> GETGQLIKDTIKNTVENTVESTHSISTEATPALQAAETGATSNASDESMIETRNVVNTHGVAETSLEGFYGRAGLVAMFTTEGGIRSWYINFGKYVQLRAKLELLTYARFDVEFTIVAQVVDEQAKVKDFNVDYQVMYVPPGASAPDGQDSFQWQSSCNPSVISNTGLPPARVSVPFMSSANAYSFSYDGYIQFGDTSSSSYGILPIHYLGQLVVRTCEDLDSARLRVRIYAKPKHMRGWIPRSPRMRPYVSRFTGIYTDAPSFCVNRESITTAG;> SAEACGYSDRVAQLTLGNSTITTQEAANIVVAYGRWPSGLRDTDATAVDKPTQPGVSAERFYTLPSVQWTTSFTGHYWKLPDALSDLGLFGQNLQFHYLYRGGWAIHVQCNATKFHQGTLLVVAVPEHKIQAQSNPSFGRTNPGEAGAACQFPFTFEDGTALGNALIYPHQWINLRTNNSATLVLPYVNAIPMDSGIKHNNWTLLVIPIVPLEYAVGATTFVPITVTIAPMCTEYNGLRAAVTQ;> GCPTLYTPGSGQFLTTDDFQTPCMLPKFQPTPVIDIPGEVKNFLEVIQVESLVEINNVSGVEGVARYRIPLNVQDAMDGQIMAVRVDPGADGPMQSTLLGVFTRYYTQWSGSLDFTFMFCGTFMTTGKVIIAYTPPGGDQPGSRQQAMLGTHVVWDFGLQSSITLVVPWISSGHFRGTSLDNTIYKYRYYEAGYITMWYQTNMVVPPNFPTEASILMFVAAQPNFSLRILKDRPDITQVASLQ;> MGAQLSKNTAGSHTTGTYATGGSSIHYTNINYYENAASNSLNKQDFTQDPDKFTRPVADIMKEAAVPLKSP

Enteroviruses (EVs) form the largest genus within the Picornaviridae family and are one of the most widespread viruses infecting animals. During the viral lifecycle, the capsid precursor domain (P1) is cleaved into VP0, VP1 and VP3 which assemble into a protomer, the fundamental subunit capable of assembling into an icosahedral capsid. Following genome encapsidation, VP0 is further cleaved into VP2 and VP4 forming the mature capsid, with VP1–VP3 responsible for forming the outer surface, while VP4 lines the internal surface of the capsid. Here, we characterize the capsid structure from a possum enterovirus W6, classified as EV-F4, a recently isolated enterovirus from the Australian brushtail possum (Trichosurus vulpecula).

We used cryo-EM to reconstruct the map of the EV-F4 capsid at a resolution of 2.96 Å and build an atomic model. The quality of the cryo-EM map enabled us to build an atomic model for EV-F4 for residues 10 to 274 of VP1, 9 to 244 of VP2, 1 to 243 to VP3, and 30 to 68 of VP4. The structure has the usual picornavirus architecture, with the three major capsid proteins having a similar β-barrel fold with the following two β-sheets, each formed by four β-strands: BIDG and CHEF, while VP4 is located along the interior of the capsid. EV-F4 loops, as for EV-E1 and EV-F3, are shorter giving the capsid a much smoother appearance. Shortening of VP1 BC and DE loops in EV-F4 and EV-F3, but also in EV-A71 results in circular 5-fold mesas that remains open in the middle instead of the occluded star-shaped mesas found in poliovirus. In both EV-F4 and EV-F3 the VP3 GH loop insertion extends into the canyon between the tip of the 3-fold propellers and the 5-fold mesas. EV-F4 does not display any charged residues in the canyon region, while the corresponding region in EV-F3 is slightly negatively charged. Interestingly, in EV-F4, the north rim of the canyon has a prominent patch of positively charged residues, which is reduced in EV-F3 and further reduced in EV-E1. We modelled this fatty acid as a sphingosine, similar to the models of EV-F3 and EV71. In EV-F4, His208 replaces Asn208 in EV-F3 and -E1 as well as in the majority of EVs, introducing a charged residue in proximity to the head of the fatty acid pocket factor.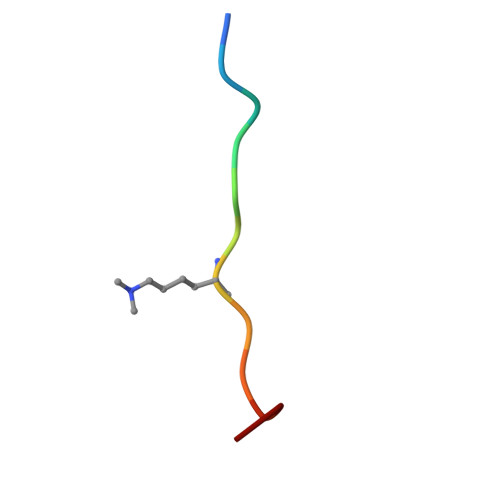> GAKRHRKVLRDN> GIVIPPQEQITQHGSPYGRCANKTRALTVAELRGSG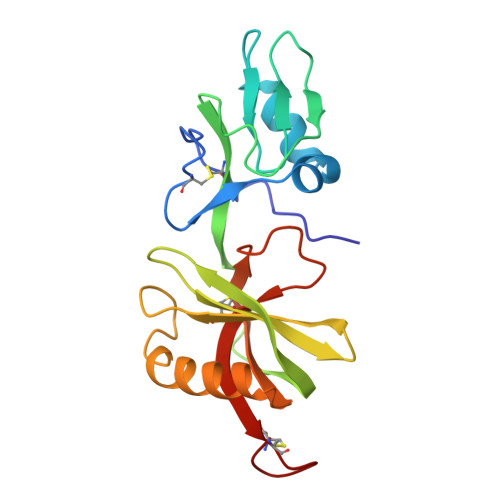DLQEYLRHVTRGWSIFALYDGTYLGGEYGGVIKDGTPGGAFDLKTTFCIMTTRNTGQPATDHYYSNVTATRLLSSTNSRLCAVFVRSGQPVIGACTSPYDGKYWSMYSRLRKMLYLIYVAGISVRVHVSKEEQYYDYEDATFETYALTGISICNPGSSLC> 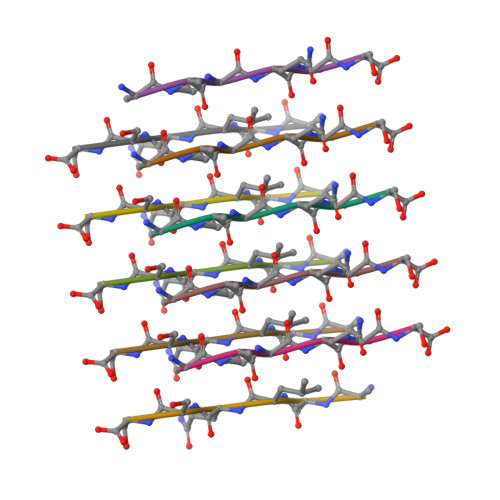AALQSS> GLLQGRMEISNSVLKTLSGFKDVYAQMNNFLQQTTDESRRMLKDAIVTQKEVLAETAAQVAGGNGEDELAAAIAATSDIETRIDGLWTLHEGEQKLRAETRADLERLAAEQAKINEEANRLQYAVRKDENAAKTMLRNAEKLMRASRFYAEFATEVSGAITVEEKLKVAEGHFPAIGRTQRDIFVLLPKGEKSLAETVNSASGAIGALIKTPPGPETLAGLSKYVDRFRTASFRLE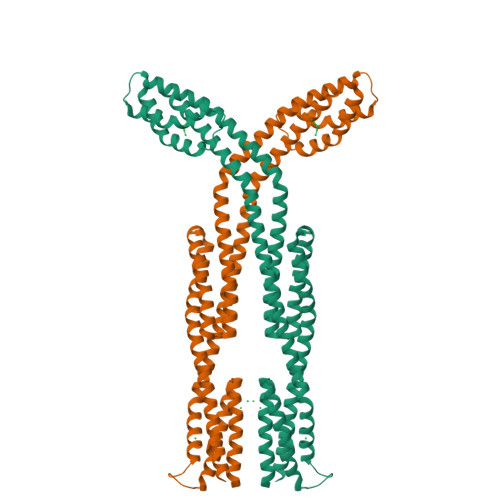AASVGKMREATQIFSELDGKIAGTESVLTATRRLSTSLTDIQIAAAAFLGTTSEESRKKLLDRFLAVQSNLTTLRGIASGMSFFDQAAGALLPIIDGMKKDGLALVEITDKRTVEFEAAGAAINEIWSDLTGFAEQQKVAAGSERAEANQ HEXANOYL-COENZYME A | C27 H46 N7 O17 P3 S 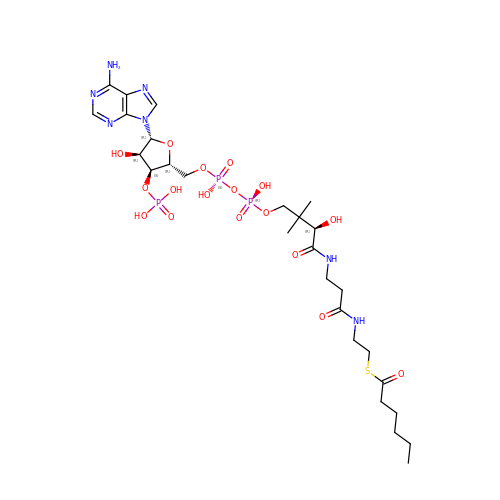| OEXFMSFODMQEPE-HDRQGHTBSA-N> MSGGFLRDDHLEFALHLHRRLAEAVPDGEVIWSPYSVACALGVLAAGARATTRTELTTLLGTDPAPLLAALDRAVTDSPDLASRTVLWVSADVPVRSSFRATMHDRPDSDVRTADFRTNPEGVRATVNADIADATRGMIRELLPQGAVTP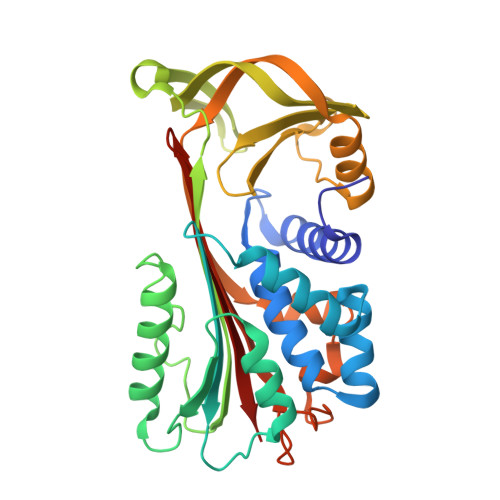DLRAILTNALWAKARWTTPFEAHLTREGTFRTPRGPKRVPFMHRTKTMPYATARGWRMVTLHAHDELAVDVLLPPGTNAAAVPTAPLLTALHRRSASTSVELALPRFELTQPHQLVEVLAEAGVRTLFTASADLSGISTVPLYVDTVIHQARLRVDERGAEGAAATAAMMLLA> LSEEQQH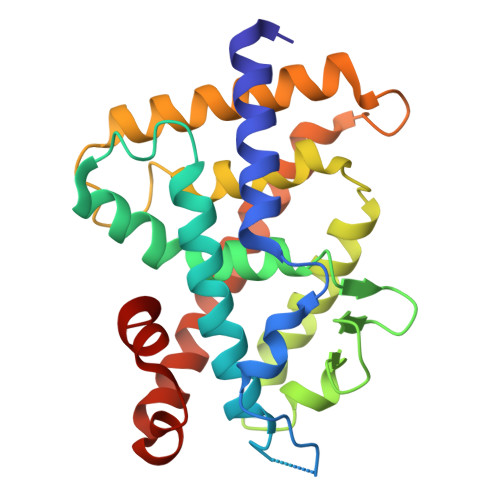IIAILLDAHHKTYDPTYADFRDFRPPVRMDGSTGSVTLDLSPLSMLPHLADLVSYSIQKVIGFAKMIPGFRDLTSDDQIVLLKSSAIEVIMLRSNQSFTMDDMSWDCGSQDYKYDVTDVSKAGHTLELIEPLIKFQVGLKKLNLHEEEHVLLMAICIVSPDRPGVQDAKLVEAIQDRLSNTLQTYIRCRHPPPGSHQLYAKMIQKLADLRSLNEEHSKQYRSLSFQPENSMKLTPLVLEVFG> APGDPRECPGLLKGVYQSEHLFESDHQSGAWCKDPLQASDKIYYMPWTPYRTDTLTEYSSKDDFIAGRPTTTYKLPHRVDGTGFVVYDGALFFNKERTRNIVKFDLRTRIKSGEAIIANANYHDTSPYRWGGKSDIDLAVDENGLWVIYATEQNNGKIVISQLNPYTLRIEGTWDTAYDKRSASNAFMICGILYVVKSVYEDDDNEATGNKIDYIYNT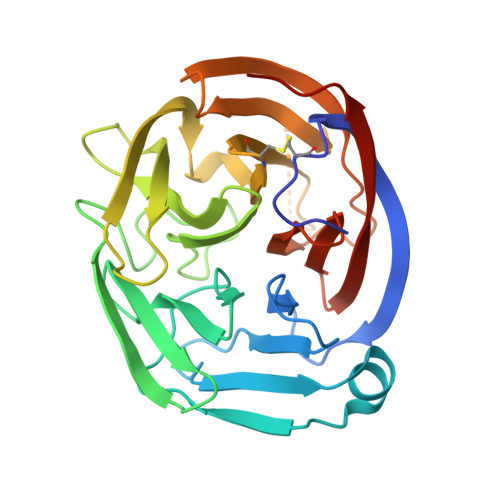DQSKDSLVDVPFPNSYQYIAAVDYNPRDNLLYVWNNYHVVKYSLDFGPAAAHHHHHHH> LTNPSQ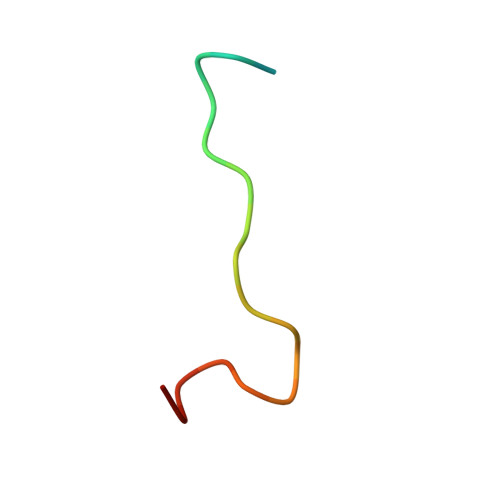YLLQDAVTEREVLLVP Proteins of the RRNPPA family are the most frequent pheromone receptors in Bacillota and use small secreted oligopeptides as pheromones. While most members of the RRNPPA family act as transcriptional factors through DNA binding, Rap receptors are specialized members that exhibit the capability to develop their function by interaction with specific protein targets. Binding of the pheromone produced from the propeptide, which is named Phr in this RRNPPA subfamily, induces Rap receptor inhibition. Our results reveal that distinct maturation processes generate multiple mature pheromones, which bind to receptors with varying affinities but produce identical structural and biological responses.

The first candidate corresponds to the canonical C-terminal peptide of 6 residues with the sequence SRGHTS and a second potential candidate would correspond to an internal pseudo-repetition of 6 residues, RRGHTA, separated by 14 amino acids. These 2 putative mature peptides only differ in the amino acids at their ends (positions 1 S/R and 6 S/A), maintaining the conserved RGHT central part of the pheromone. Interestingly, the internal pheromone RRGHTA showed the highest stabilization with a dTm of 75°C while the canonical C-terminal hexapeptide pheromone showed a much lower (63°C) dTM. Rap3T shows 4 times lower affinity (EC50 20,75 nM) for the putative Phr3T C-terminal canonical pheromone (SRGHTS) and more than 10 times lower affinity (EC50 69,75 nM) for the possible maturation variant of this peptide with one less amino acid. To molecularly assess the differences in affinity and stabilization for the alternative peptides analyzed we solved the structures for Rap3T in complex with RRGHTAS, SRGHTS, and RGHTS. Rap complexes with RRGHTA and SRGHTS peptides displayed C2221 space group and with cell dimensions that only allowed the presence of 1 monomer in the asymmetric unit generating the dimer by crystallographic symmetry. Remarkably, these structures exhibited nearly identical conformations as confirmed by the low differences in the superimposition of their Cα atoms for either individual monomers or the complete dimers (RMSD 0.36–0.50), dispelling the notion of peptides eliciting divergent conformational shifts. Comparison of complexes with RRGHTA and SRGHTS peptides showed that the sidechain of Arg in position 1 for RRGHTA mediates a network of salt-bridges with D264 and D335 plus hydrophobic interactions with M304 meanwhile the Ser in this position for SRGHTS only makes a hydrogen bound with Y225. These differences in interactions for position 1 may explain the lower stabilization seen in thermal shift assays and the higher EC50 value from thermophoresis assays for SRGHTS. In contrast, at the C-terminal end, the presence of a Ser in the SRGHTS peptide does not excessively broaden the interactions of Ala in the RRGHTA peptide.

> MLEQMISSSKVGVKINEWYKYIRLFSVPDSEILKAEVEEEIRHMKEDHDLLLYYSLMCFRHQLMLDYLEPKTLNEERPKISDLLEKIESSQTDLKGILEYYFNFFRGMYEFEQYEYLNAISFYKQAERKLSLVADEIERAEFHYKVAEIYYHMKQTHMSMHHIVQAIDSYKAHENYTVRVIQCSFVIGLNYLDMDYPEKAIPHFKNALDKAREIDMSRLIGSSLYNLGLCSFAEEAYEKASEYFKEGIRVYQDNGYEHSNRILDILLMLTKTTFKMRNHSEGISWCAHGLSLSKNLNDEIMAKMFEFIHALYVDNDNEKLNSILNYLELKSMLSDVEDLASDAAKYYNEKEDHKVAVAYYEKVLYARKQIQRGDCLYET;> SRGHTS>KEEEDVICDGCNGPVVGTRY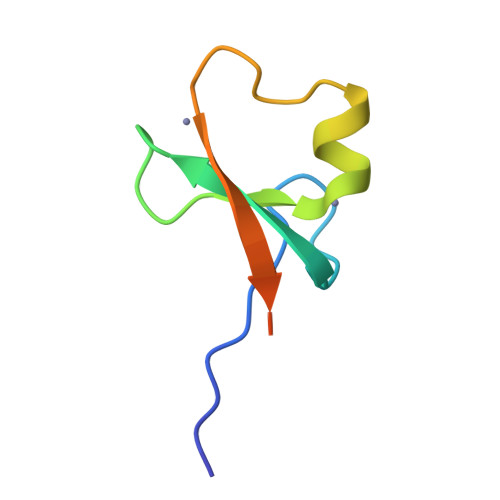KCSVCPDYDLCSVCEGKGLHRGHTKLAFPSPFGHLSEGFS[2x]>[2x]MISMKPRYKPDWESLREHTVPKWFDKAKFGIFIHWGIYSVPGWATPTGELGKVPMDAWFFQNPYAEWYENSLRIKESPTWEYHVKTYGENFEYEKFADLFTAEKWDPQEWADLFKKAGAKYVIPTTKHHDGFCLWGTKYTDFNSVKRGPKRDLVGDLAKAVREAGLRFGVYYSGGLDWRFTTEPIRYPEDLSYIRPNTYEYADYAYKQVMELVDLYLPDVLWNDMGWPEKGKEDLKYLFAYYY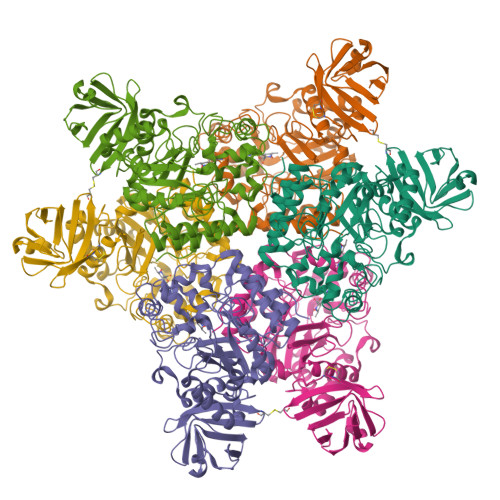NKHPEGSVNDRWGVPHWDFKTAEYHVNYPGDLPGYKWEFTRGIGLSFGYNRNEGPEHMLSVEQLVYTLVDVVSKGGNLLLNVGPKGDGTIPDLQKERLLGLGEWLRKYGDAIYGTSVWERCCAKTEDGTEIRFTRKCNRIFVIFLGIPTGEKIVIEDLNLSAGTVRHFLTGERLSFKNVGKNLEITVPKKLLETDSITLVLEAVEEHHHHHH> XLAAAMAQ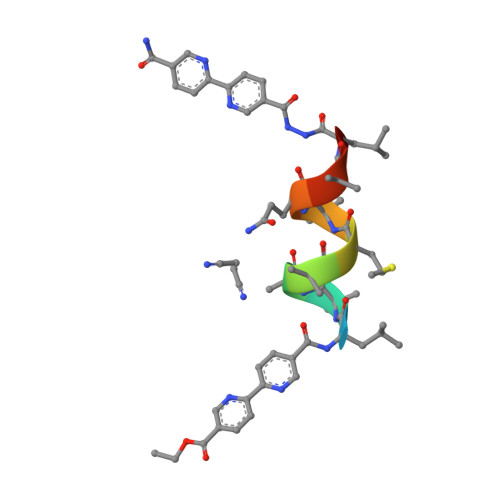ALX>MTGLTILRNANVYAPQPLGLKTVLVGGGKILAITDEALELPASIVADDIDLQGRILTPGFIDAHAHITGGGGEAGFATQVPPVPLSQFTAFGVTTVVGLLGTDDTTRSTGNLLSRVYGLREEGMSAYCWTGGYHYPLTTLMGSAREDIVYMEPIIGVGEFAISDHRSSQPQFEEVIRIASDAHVAGLMTGKAGIVHFHLGDGSRKLALIKRALAETELPARVFNPTHVNRNKPLFDEACEMLSQGIYIDITAFPDDAVDDGWSAAEALLLAKERGCPLKQITISSDGGGCMPAFDASGAVVAMDFGRSETLLATLKTVTAQGMALEDVLSSLTANVAHLLRLPAKGKIATGADADLLVLDADYSINDVMALGRWHLRDKALIMKGTFEENLYFQ[8x]

Cyanophycin is a bacterial biopolymer used for storage of fixed nitrogen. First, cyanophycinase breaks down the backbone peptide bonds, releasing β-Asp-Arg dipeptides. Then, these dipeptides are broken down into free Asp and Arg by enzymes with isoaspartyl dipeptidase activity. Two bacterial enzymes are known to have significant β-aspartyl dipeptidase activity: isoaspartyl dipeptidase (IadA), a bacterial zinc metallopeptidase; and isoaspartyl aminopeptidase (IaaA, also called plant-type asparaginase, EcAIII and IadC), a common Ntn-family enzyme with known plant and animal homologs.

LmIadA has 44% sequence identity to E. coli IadA (EcIadA32). Like EcIadA, the purified enzyme forms octamers in solution. We examined the activity of LmIadA towards several β-aspartyl dipeptides and found that it displayed no apparent preference towards β-Asp-Arg/Lys. To confirm the structural basis for this lack of specificity, we solved the structure of the wild type enzyme at 1.8 Å resolution and compared it to that of EcIadA32. The crystal structure of LmIadA shows a homooctameric architecture as the asymmetric unit. Two Zn2+ ions are liganded by H64, H66, H198, H227 and E159, corresponding to EcIadA H68, H70, H201, H230 and carboxylated K162. Substrate binding residues in EcIadA such as E77, T106 and R23332, are also present at corresponding positions in LmIadA (E73, T102 and R230) and display similar conformations. The loop formed by LmIadA T251-Y262 is longer and bulkier than the corresponding one of EcIadA (S255-V261), and as a result could restrict access to the active site. However, the partially flexible region between G288-G306 (EcIadA G288-G303) is oriented away from the binding pocket. This leads to a similarly sized opening in the active site region surrounding the non-Asp portion of the substrate and explains the lack of specificity.> HHHHHHMAILTDENYVDKAERAISLLEKDNKGNYLLTTSQIRKLLSLCSSLYDR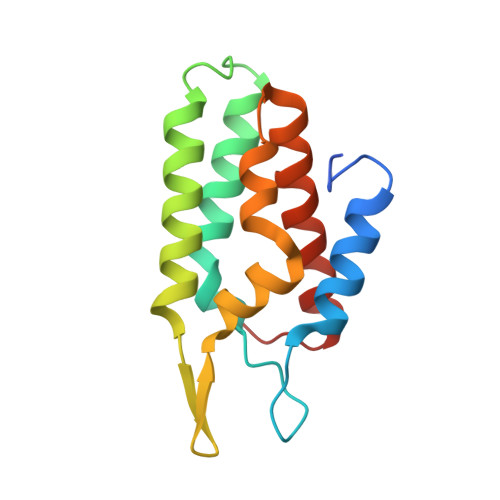SKERKFDELINDVSYLRVQFVYQSGRNSVRVNRQTFFPVKDLVEKGQILEALKEIKDRETLQRFCRYMEALVAYFKFYGGKD>MAAQQCNGIYIWKIGNFGMHLKCQEEEKPVVIHSPGFYTGKPGYKLCMRLHLQLPTAQRCANYISLFVHTMQGEYDSHLPWPFQGTIRLTILDQSEAPVRQNHEEIMDAKPELLAFQRPTIPRNPKGFGYVTFMHLEALRQRTFIKDDTLLVRCEVSTRFDLEHHHHHH[2x];>[2x]GPCH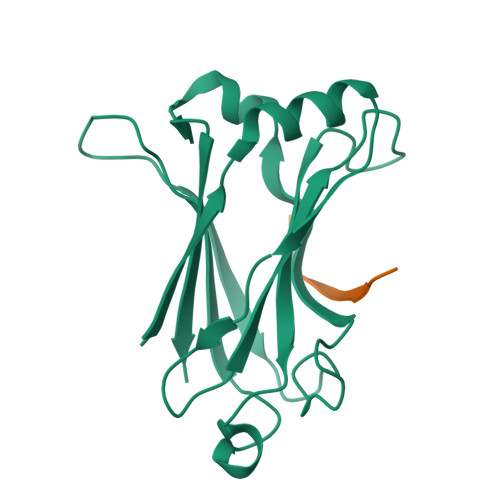GPEENEYKSEGTFGI> MNFIQYIDDSYAVKVKEI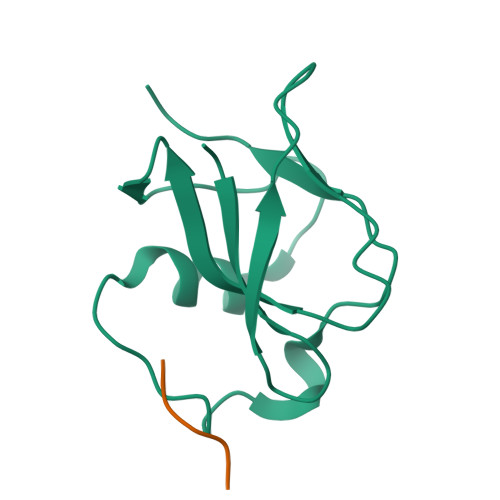NSSEGFYINGIQTPFFILSVFIGNKRVTGVEFNNYDSLPMLSVINDLGNIDLNVIPQNYFATAFTEIYFNIPF> MSTRPKISLIVAALQPSMGIGAKGSLPWRLKNEMKYFKDVTSKAKDGHINAVVMGRKTWELIPERFRPLAGRLNVILSRKNDDLIDSNGVYHFSSFDSVMKHLEKD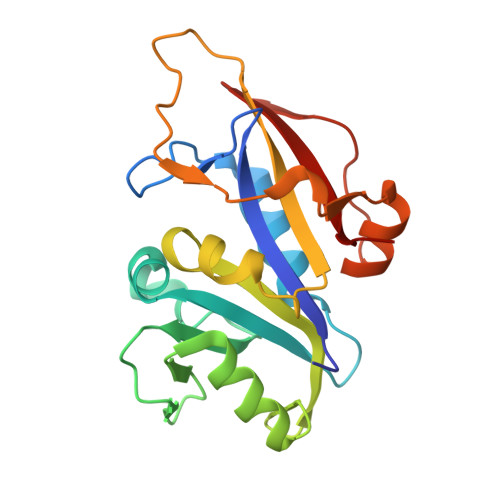SFRFKDMPLDKIFIIGGSQIYNLLILDSRVDNLLVTQVHFVGEDADKPQMDTFLDWDLSKWKRLEHDKLEQYVGLDVPRGLNEEGSYNYEYTMWEKAQ> GHMDEISETNTIFKLEGVSVLSPLRKKLDLVFYLSNVDGSPVITLLKGNDRELSIYQLNKNIKMASFLPVPEKPNLIYLFMTYTSCEDNKFSEPVVMTLNKENTLNQFKKLGLLDSNVTDFEKCVEYIRKQAILTGFKISNPFVNSTLVDTDAEKINSFHLQCHRGTKEGTLYFLPDHIIFGFKKPILLFDASDIESITYSSITRLTFNASLVTKDGEKYEFSMIDQTEYAKIDDYVKRK;> MRDSTECQRIIRRGVNCLMLPKGMQRSSQNRSKWDKTMDLFVWSVEWILCPMQEKGEKKELFKHVSHRIKETDFLVQGMGKNVFQKCCEFYRLAGTSSCIEGEDGSETKEERTQILQKSGLKFYTKTFPYNTTHIMDSKKLVELAIHEKCIGELLKNTTVIEFPTIFVAMTEADLPEGYEVLHQE

Biogenesis of eukaryotic box C/D small nucleolar ribonucleoproteins initiates co-transcriptionally and requires the action of the assembly machinery including the Hsp90/R2TP complex, the Rsa1p:Hit1p heterodimer and the Bcd1 protein. We show that Bcd1p binds Rtt106p and controls its transcription-dependent recruitment by reducing its association with RNA polymerase II, modulating H3K56ac levels at gene body. We reveal the 3D structures of the free and Rtt106p-bound forms of Bcd1p using nuclear magnetic resonance and X-ray crystallography. Bcd1p interacts with a region that is distinct from the interaction interface between the histone chaperone and histone H3.

To understand the mode of interaction of Bcd1p120-303 with Rtt106p65-301, we characterized the 3D structure of the complex using X-ray crystallography. The final structure was refined against the dataset collected from a native crystal to an Rfactor of 21.0% and an Rfree of 29.7%, including all reflections between 20 and 2.79 Å resolution. The asymmetric unit contains one Bcd1p120-303:Rtt106p65-301 heterodimer. The three loops in bound Bcd1p encompassing residues 173–177, 211–224, and 248–252, respectively, were not built due to the lack of density explained by their high flexibility in their native free state. Indeed, the two 3D structures closely resembled one another and 3D superimposition revealed that no significant conformational modifications of Bcd1p120–303 occurred upon binding to Rtt106p65–301. We concluded that the conformational changes induced by complex formation mostly occurred in Rtt106p. The crystal structure of the Bcd1p120–303:Rtt106p65-301 complex revealed that Rtt106p interacts with Bcd1p only via its PH1 domain. Most of the residues from Rtt106p that are buried upon interaction with Bcd1p are located in two distinct parts, including residues of the first S1 and S2 β-strands, solvent-exposed residues from the contiguous α-helices H1 and H2, and residues from the loop connecting these two α-helices. For Bcd1p, the interaction interface mainly involved the solvent-exposed faces of helix α1 and of strand β6 located on one edge of the central β-strand. A hydrophobic cluster formed at the heterodimer interface with side-chain interactions of four hydrophobic residues from each protein.> MGSHQERPLIGLLFSETGVTADIERSQRYGALLAVEQLNREGGVGGRPIETLSQDPGGDPDRYRLCAEDFIRNRGVRFLVGCYMSHTRKAVMPVVERADALLCYPTPYEGFEYSPNIVYGGPAPNQNSAPLAAYLIRHYGERVVFIGSDYIYPRESNHV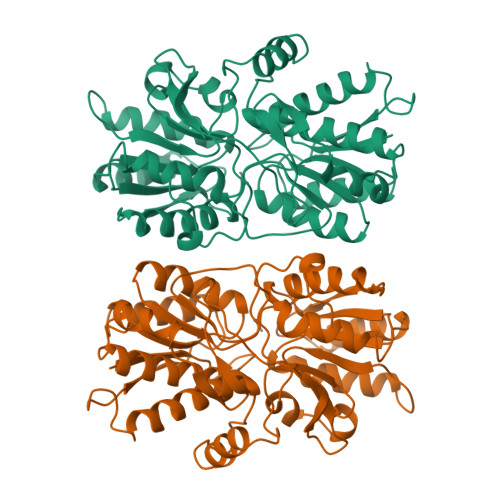MRHLYRQHGGTVLEEIYIPLYPSDDDLQRAVERIYQARADVVFSTVVGTGTAELYRAIARRYGDGRRPPIASLTTSEAEVAKMESDVAEGQVVVAPYFSSIDTPASRAFVQACHGFFPENATITAWAEAAYWQTLLLGRAAQAAGNWRVEDVQRHLYDIDIDAPQGPVRVERQNNHSRLSSRIAEIDARGVFQVRWQSPEPIRPDPYVVVHNLDDWSASMGGGPLP> MKKLYIITGPAGVGKSTTCKRLAAQLDNSAY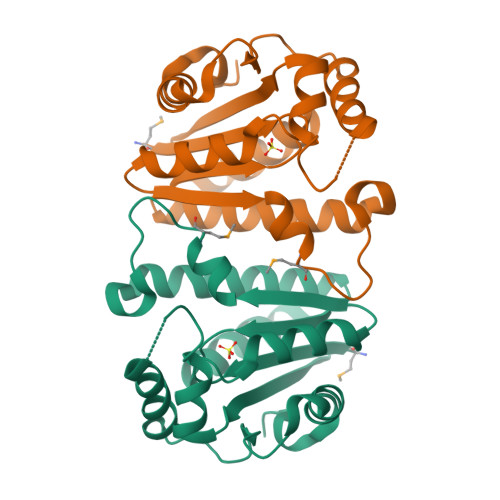IEGDIINHMVVGGYRPPWESDELLALTWKNITDLTVNFLLAQNDVVLDYIAFPDEAEALAQTVQAKVDDVEIRFIILWTNREELLRRDALRKKDEQMGERCLELVEEFESKGIDERYFYNTSHLQPTNLNDIVKNLKTNPRFIFCMAGDPLEHHHHHH> SDKGKLSLQDVAELIRARACQRVVVMVGAGISTPSGIPDFRSPGSGLYSNLQQYDLPYPEAIFELPFFFHNPKPFFTLAKELYPGNYKPNVTHYFLRLLHDKGLLLRLYTQNIDGLERVSGIPASKLVEAHGTFASATCTVCQRPFPGEDIRADVMADRVPRCPVCTGVVKPDIVFFGEPLPQRFLLHVVDFPMADLLLILGTSLEVEPFASLTEAVRSSVPRLLINRDLVGPLAWHPRSRDVAQLGDVVHGVESLVELLGWTEEMRDLVQRETGKLDGPDK;> SYGRKKRRQ

Sirtuins are NAD+-dependent protein lysine deacylases implicated in metabolic regulation and aging-related dysfunctions. Sirt1 features the conserved sirtuin catalytic core of ~270 residues, which comprises a Rossman-fold domain and a smaller Zn2+-binding module. A cleft between these subdomains accommodates NAD+ and recognizes the acylated substrate polypeptide with low sequence selectivity, and binding of these substrates is accompanied by Sirt1 closure movements. Tat binds to the sirtuin catalytic core and inhibits Sirt1, Sirt2, and Sirt3 with comparable potencies.

To analyze why Tat inhibits sirtuins instead of serving as a regular substrate, we solved the crystal structure of a Sirt3/ac-Tat-46–54 complex at 1.65 Å resolution and refined it to Rcryst/Rfree values of 18.1/20.9%. Residues 46–54 of the Tat substrate peptide are inserted in the substrate binding groove in the typical, β-sheet-like fashion observed in a previous Sirt1/ac-p53 peptide complex and other sirtuin/substrate complexes. The acetylated Tat Lys50 interacts with Sirt3 Val292, Phe293/294, and the catalytic His248, and comparable interactions would be formed with Sirt1. In addition, Tat residues in the range of (−3) to (+3) relative to Lys50 interact, similarly, with Sirt3 (and likely Sirt1) in the complexes with acetylated and non-acetylated Tat, respectively. Small differences in this range concern sidechain conformation, which does not affect directed interactions. Larger differences are seen for more remote residues, Ser46 at the N-terminus, and Gln54 at the C-terminus and indicate a different chain orientation from there on. In particular, the binding mode of the more C-terminal Tat residues comprising the basic region, which seems to be key in inhibitory Tat binding, could be influenced electrostatically by Lys50 acetylation, which removes a positive charge. Using ac-Tat-46–54 as a substrate revealed efficient Sirt1-dependent deacetylation, even slightly more efficient than for its standard substrate peptide ac-p53-Lys382. Our data, indeed, indicate that Tat binds in a slightly different conformation compared to a substrate and that Tat serving as a substrate has to dissociate before it can bind in the inhibitory mode.>SMQEEDTFRELRIFLRNVTHRLAIDKRFRVFTKPVDPDEVP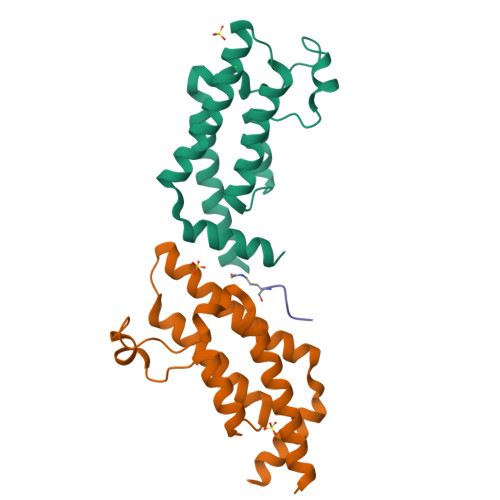DYVTVIKQPMDLSSVISKIDLHKYLTVKDYLRDIDLICSNALEYNPDRDPGDRLIRHRACALRDTAYAIIKEELDEDFEQLCEEIQESR[2x];> STGGK N,N-diethyl-2-methylpyrimidine-4-carboxamide | C10 H15 N3 O | 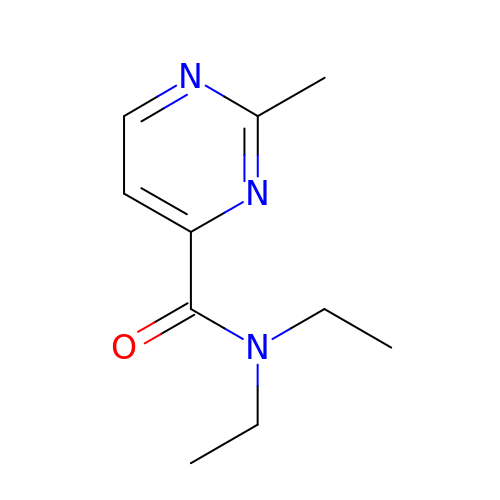MBLSTDCRYDGJKF-UHFFFAOYSA-N> MAGTSGLLNAVKP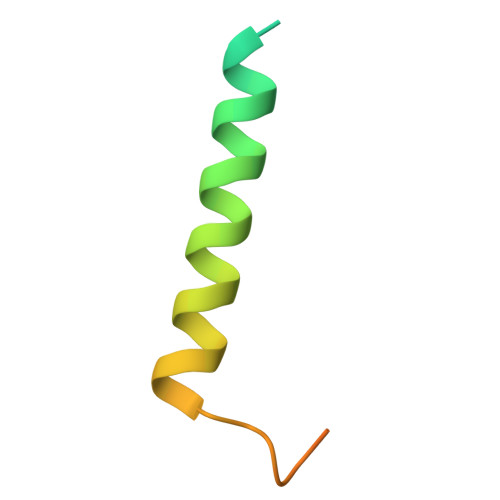KIQTIDIQAAAGWGIAAAAGAIWVVQPFGWIKKTFIDPPPTEEK> M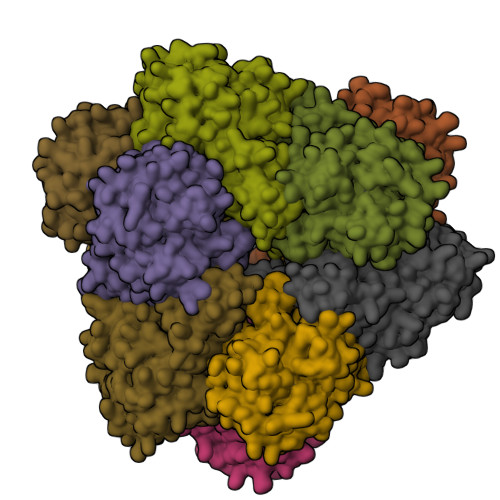EVRNMVDYELLKKVVEAPGVSGYEFLGIRDVVIEEIKDYVDEVKVDKLGNVIAHKKGEGPKVMIAAHMDQIGLMVTHIEKNGFLRVAPIGGVDPKTLIAQRFKVWIDKGKFIYGVGASVPPHIQKPEDRKKAPDWDQIFIDIGAESKEEAEDMGVKIGTVITWDGRLERLGKHRFVSIAFDDRIAVYTILEVAKQLKDAKADVYFVATVQEEVGLRGARTSAFGIEPDYGFAIDVTIAADIPGTPEHKQVTHLGKGTAIKIMDRSVICHPTIVRWLEELAKKHEIPYQLEILLGGGTDAGAIHLTKAGVPTGALSVPARYIHSNTEVVDERDVDATVELMTKALENIHELKI Carboxysomes are anabolic BMCs for autotrophic CO2 fixation found in all cyanobacteria and many proteobacteria. The carboxysome is composed of a polyhedral shell that encapsulates the key CO2-fixation enzyme, ribulose-1,5-bisphosphate carboxylase/oxygenase (Rubisco), and carbonic anhydrase (CA), which dehydrates HCO3− to CO2, the substrate for Rubisco carboxylation. In α-carboxysomes, the disordered linker protein CsoS2 plays an essential role in carboxysome assembly and Rubisco encapsulation. In this work, we synthetically engineer α-carboxysome shells using minimal shell components derived from a chemoautotroph Halothiobacillus (H.) neapolitanus, a model system in the fundamental studies and synthetic engineering, and determine high-resolution cryoEM structures of the shells of variable constituents.

The high-quality map of the T = 9 shell (1.86 Å resolution) allows for accurate modelling of CsoS2-C that tightly associates with shell proteins, resulting in an atomic model of the T = 9 shell comprising 80 CsoS1A hexamers, 12 CsoS4A pentamers and 60 CsoS2-C. Of those, interfaces 3 and 4 are unique to the T = 9 shell, whereas interfaces 1 and 2 are present in all three shells as previously reported. In contrast, the angles between two hexamers in interfaces 3 and 4 are arranged in a planar fashion, markedly different from those in interfaces 1 and 2, and also different from those measured in other BMC mini-shells. The cryoEM structure of the T = 9 shell at 1.86 Å resolution enables the characterization of CsoS2 and its interactions with the shell at atomic details. It is clearly well-resolved for the most of C-terminus in the cryoEM map, allowing unambiguous assignment of amino acid residues of three fragments of CsoS2-C: F1, Arg712−Arg731; F2, Leu773−Gly823; F3, Glu829−Gly869. The cryoEM structure revealed that the F1, F2, F3 fragments adopt completely different conformations from the AlphaFold2-predicted structures. They form extensive hydrogen bonds and salt bridges with both CsoS1A and CsoS4A at three distinct binding sites, with the surface contact area of 767.1, 3333.0, and 1851.7 Å2, respectively. Interestingly, all three CsoS2-C fragments, F1 to F3, bind specifically to the tri-capsomere interfaces. While CsoS2-F1 and F2 interact with three CsoS1A hexamers, CsoS2-F3 acts on the interface between one CsoS4A pentamer and two CsoS1A hexamers, with the extreme C-terminus buried inside the cavity formed by the interface. The three CsoS2-C F1-F3 fragments associate tightly with shell proteins simultaneously and essentially “stitches” the capsomeres together at the inner surface of the T = 9 shell. However, a close inspection of the interfaces uncovers a common interaction motif among these interactions: alignment of all the CsoS1A-CsoS2 interfaces identifies a repetitive Ile(Val)-Thr-Gly ([IV]TG) motif that interacts with the β-strand of highly conserved CsoS1A through His79 and hydrogen bonds in the main chain.

>MADVTGIALGMIETRGLVPAIEAADAMTKAAEVRLVGRQFVGGGYVTVLVRGETGAVNAAVRAGADACERVGDGLVAAHIIARVHSEVENILPKAPQA[8x];> MKIMQVEKTLVSTNRIADMGHKPLLVVWEKPGAPRQVAVDAIGCIPGDWVLCVGSSAAREAAGSKSYPSDLTIIGIIDQWNGE;> MNPADLSGLSGKELARARRAALSKQGKAAVSNKTASVNRSTKQAASSINTNQVRSSVNEVPTDYQMADQLCSTIDHADFGTESNRVRDLCRQRREALSTIGKKAVKTNGKPSGRVRPQQSVVHNDAMIENAGDTNQSSSTSLNNELSEICSIADDMPERFGSQAKTVRDICRARRQALSERGTRAVPPKPQSQGGPGRNGYQIDGYLDTALHGRDAAKRHREMLCQYGRGTAPSCKPTGRVKNSVQSGNAAPKKVETGHTLSGGSVTGTQVDRKSHVTGNEPGTCRAVTGTEYVGTEQFTSFCNTSPKPNATKVNVTTTARGRPVSGTEVSRTEKVTGNESGVCRNVTGTEYMSNEAHFSLCGTAAKPSQADKVMFGATARTHQVVSGSDEFRPSSVTGNESGAKRTITGSQYADEGLARLTINGAPAKVARTHTFAGSDVTGTEIGRSTRVTGDESGSCRSISGTEYLSNEQFQSFCDTKPQRSPFKVGQDRTNKGQSVTGNLVDRSELVTGNEPGSCSRVTGSQYGQSKICGGGVGKVRSMRTLRGTSVSGQQLDHAPKMSGDERGGCMPVTGNEYYGREHFEPFCTSTPEPEAQSTEQSLTCEGQIISGTSVDASDLVTGNEIGEQQLISGDAYVGAQQTGCLPTSPRFNQTGNVQSMGFKNTNQPEQNFAPGEVMPTDFSIQTPARSAQNRITGNDIAPSGRITGPGMLATGLITGTPEFRHAARELVGSPQPMAMAMANRNKAAQAPVVQPEVVATQEKPELVCAPRSDQMDRVSGEGKERCHITGDDWSVNKHITGTAGQWASGRNPSMRGNARVVETSAFANRNVPKPEKPGSKITGSSGNDTQGSLITYSGGARG>[2x]MEDAKNIKKGPAPFYPLEDGTAGEQLHKAMKRYALVPGTIAFTDAHIEVNITYAEYFEMSVRLAEAMKRYGLNTNHRIVVCSENSLQFFMPVLGALFIGVAVAPANDIYNERELLNSMNISQPTVVFVSKKGLQKILNVQKKLPIIQKIIIMDSKTDYQGFQSMYTFVTSHLPPGFNEYDFVPESFDRDKTIALIMNSSGSTGLPKGVALPHRTACVRFSHARDPIFGNQIIPDTAILSVIPFHHAFGMSTTLGYLICGFRVVLMYRFEEELFLRSLQDYKIQSALLVPTLFSFFAKSTLIDKYDLSNLHEIASGGAPLSKEVGEAVAKRFHLPGIRQGYGLTETTSAILITPEGDD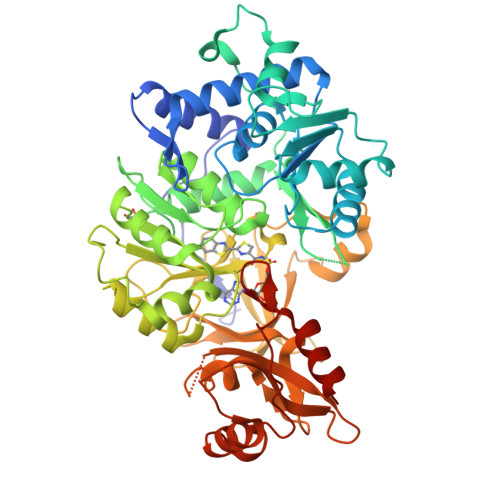KPGAVGKVVPFFEAKVVDLDTGKTLGVNQRGELCVRGPMIMSGYVNNPEATNALIDKDGWLHSGDIAYWDEDEHFFIVDRLKSLIKYKGYQVAPAELESILLQHPNIFDAGVAGLPDDDAGELPAAVVVLEHGKTMTEKEIVDYVASQVTTAKKLRGGVVFVDEVPKGLTGKLDARKIREILIKAKKGGKSKL{(3R)-3-[(2-methoxyphenyl)methyl]morpholin-4-yl}[3-(4-methylpyridin-2-yl)-1H-pyrazol-5-yl]methanone | C22 H24 N4 O3 | 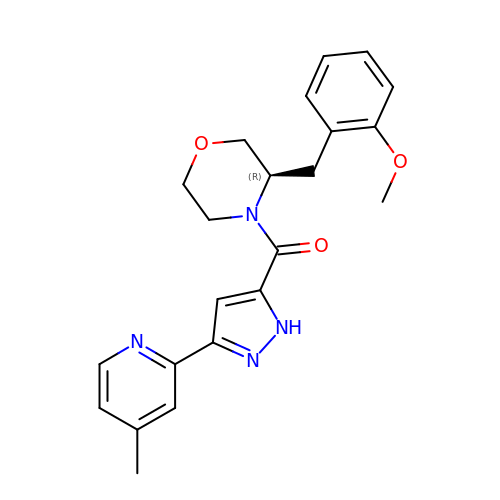FTBXWZMCYGGBTG-QGZVFWFLSA-N> SPPAVPQTFQVAHLHAPTGSGKSTKVPAAYAAQGYKVLVLNPSVAATLGFGAYMSKAHGIDPNIRTGVRTITTGAPITYSTYGKFLADGGCSGGAYDIIICDECHSTDSTTILGIGTVLDQAETAGARLVVLATATPPGSVTVPH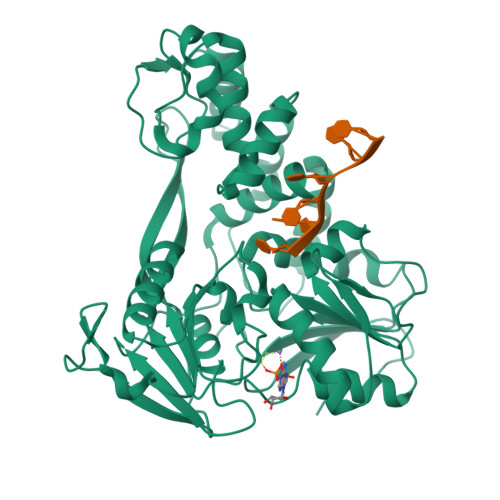PNIEEVALSSTGEIPFYGKAIPIETIKGGRHLIFCHSKKKCDELAAKLSGLGLNAVAYYRGLDVSVIPTSGDVIVVATDALMTGFTGDFDSVIDCNTCVTQTVDFSLDPTFTIETTTVPQDAVSRSQRRGRTGRGRMGIYRFVTPGERPSGMFDSSVLCECYDAGCAWYELTPAETSVRLRAYLNTPGLPVCQDHLEFWESVFTGLTHIDAHFLSQTKQAGDNFPYLVAYQATVCARAQAPPPSWDQMWKCLIRLKPTLHGPTPLLYRLGAVQNEVTTTHPITKYIMACMSA>GPHMADLSIILSKSQLQDTLIHLIKNDSSFLSTLHEVYLQVL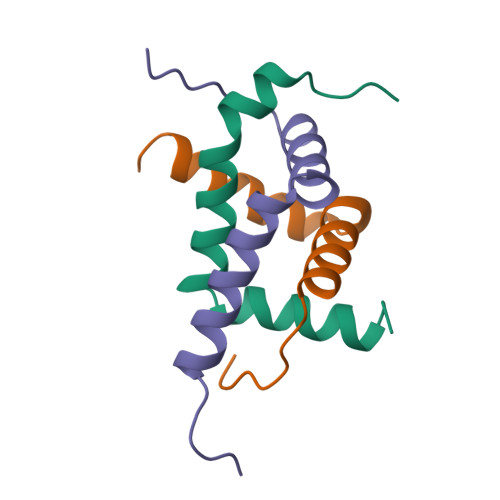TKNKDNHNL[3x]> SMEEVGKGGQSAKFVTYSTSEPAKLFGEAGRRSHFRARVLEATLSPLEKAIFDVPIEEWLTVDRSKFSGWRCAVPHPVTADELKPVDSSHDILRHIALYNGPVTDLQLDA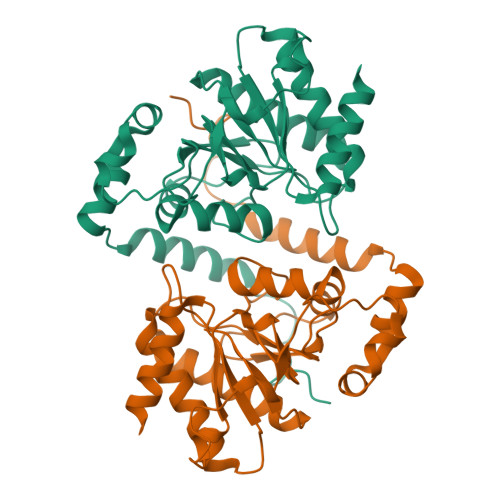IVNAANKTCLGGKGVDGAIHAAAGPLLVRECATFKGCDTGQCRLTKGYNLPARYVLHTVGPIGERPEELRSCYRSILSLAHRNRLRSIGFCCVSTGVYGYPLIPATRIAVDETIEYLKQHFSAFDLCCFACFKLEEYNAYTDCLRAWLGTAPNASTDQ> GIDPFTMATFISVQ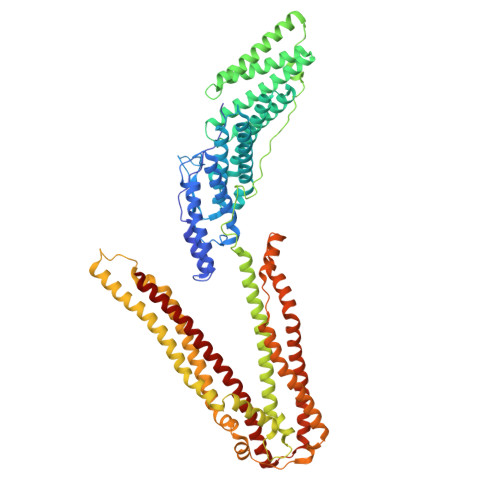LKKTSEVDLAKPLVKFIQQTYPSGGEEQAQYCRAAEELSKLRRAAVGRPLDKHEGALETLLRYYDQICSIEPKFPFSENQICLTFTWKDAFDKGSLFGGSVKLALASLGYEKSCVLFNCAALASQIAAEQNLDNDEGLKIAAKHYQFASGAFLHIKETVLSALSREPTVDISPDTVGTLSLIMLAQAQEVFFLKATRDKMKDAIIAKLANQAADYFGDAFKQCQYKDTLPKEVFPVLAAKHCIMQANAEYHQSILAKQQYYFGEEIARLQHAAELIKTVASRYDEYVNVKDFSDKINRALAAAKKDNDFIYHDRVPDLKDLDPIGKATLVKSTPVNVPISQKFTDLFEKMVPVSVQQSLAAYNQRKADLVNRSIAQMREATTLANGVLASLNLPAAIEDVSGDTVPQSILTKSRSVIEQGGIQTVDQLIKELPELLQRNREILDESLRLLDEEEATDNDLRAKFKERWQRTPSNELYKPLRAEGTNFRTVLDKAVQADGQVKECYQSHRDTIVLLCKPEPELNAAIPSANPAKTMQGSEVVNVLKSLLSNLDEVKKEREGLENDLKSVNFDMTSKFLTALAQDGVINEEALSVTELDRVYGGLTTKVQESLKKQEGLLKNIQVSHQEFSKMKQSNNEANLREEVLKNLATAYDNFVELVANLKEGTKFYNELTEILVRFQNKCSDIVFAR>[2x]MEIEKNDYLLSANGSKAIDFVWSNFLKHPYNPKLKQPDANVKAAWEKHADWEHWSNMGQDWSLNTPSGLVPRPNHGIAHTLRVAQLVPVIAEFLKAYSGDPKFQKLTQKEIQKAQYMMLFSVIGRENDMSWTDANHYQQAFKEAYNGQYSKHIYATFKENAQKG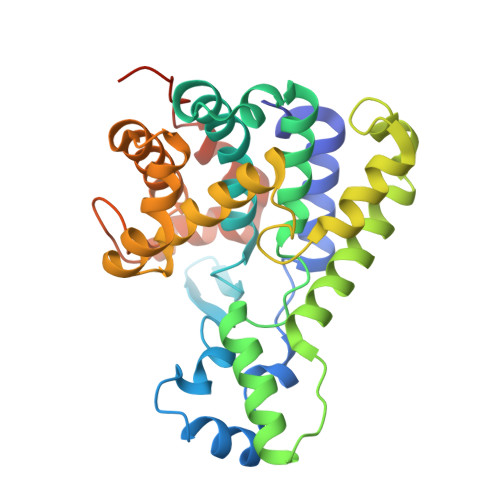FLNHVVTNKSSLIPSLFSDESELQYWAEALDTGKPGISSASGILMALAHDLDLMRCYDKGKFNSLKMKDLVARLGGNEDAAKKLADYAHDLIVATGDRCMGYGVTQDYNYSLFGKCSLDPNECLKQLQSIPKPETTLANQYGILEHHHHHH>GSANSQLVVRAKFNFQQTNEDELSFSKGDVIHVTRVEEGGWWEGTHNGRTGWFPSNY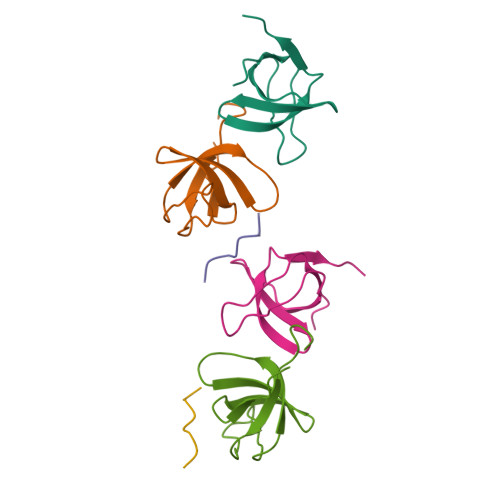VREIKPS[2x];> RPPKPRPR>[3x]TIKPVEYYKPDGCNKTNDHFTMQPGVNFYTVPNLGPSSSSADECYTNPSFSIGSSIYMFSQEIRKTDCTTGEILSIQIVLGRIVDKGQQGPQASPLLVWSVPNPKIINSCAVAAGDETGWVLCSVTLTAASGEPIPHMFDGFWLYKFEPDTEVVAYRITGFAYLLDKVYDSVFIGKGGGIQRGNDLYFQMFGLSRNRQSIKAL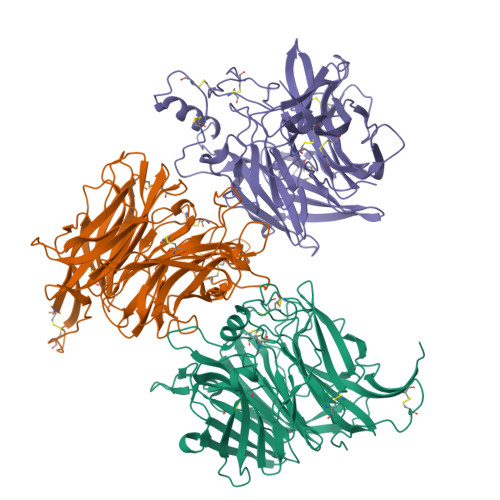CEHGSCLGTGGGGYQVLCDRAVMSFGSEESLISNAYLKVNDVASGKPTIISQTFPPSDSYKGSNGRIYTIGERYGIYLAPSSWNRYLRFGLTPDISVRSTTWLKEKDPIMKVLTTCTNTDKDMCPEICNTRGYQDIFPLSEDSSFYTYIGITPSNEGTKSFVAVKDDAGHVASITILPNYYSITSATISCFMYKEEIWCIAVTEGRKQKENPQRIYAHSYRVQKMCFNIKP(3S)-3-[(3-aminophenyl)sulfanylmethyl]piperidine-2,6-dione 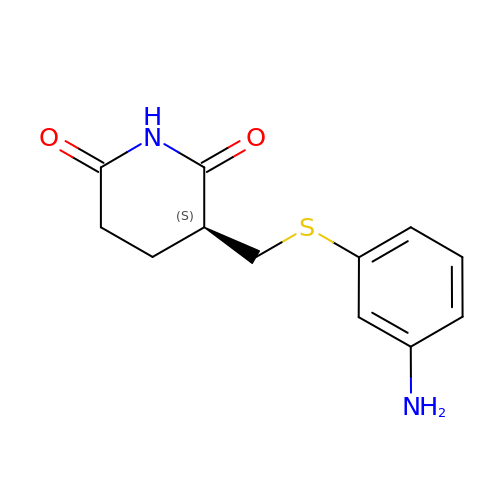| C12 H14 N2 O2 S | YGPLIXYOXPSSRZ-MRVPVSSYSA-N Several studies have identified the enzyme type I dehydroquinase (DHQ1, 3-dehydroquinate dehydratase, EC 4.2.1.10) as a promising target for anti-virulence drug development. DHQ1 catalyzes the reversible dehydratation of 3-dehydroquinic acid (1) to 3-dehydroshikimic acid (2), which is the third step in the shikimic acid pathway. It follows a covalent catalysis mechanism with the formation of transient Schiff base species´ between the ketone moiety of the substrate and the ɛ-amino group of a catalytic lysine residue (K160/K170 in Sa-DHQ1 and St-DHQ1, respectively), which are finally hydrolyzed to regenerate the enzyme. An essential histidine residue (H133/H143 in Sa-DHQ1 and St-DHQ1, respectively), is also involved in the formation/hydrolysis of the Schiff base intermediates.

Herein we report the synthesis of compounds 6–7 in which enhancement of the electrophilicity of an endocyclic carbon atom in the ligand towards covalent modification is attempted by direct introduction of the amino functionality into the quinate scaffold. These compounds are substrate analogs in which the carbonyl group at C3 has been replaced by a hydroxyamino and an amino group with R configuration (compounds 6 and 7, respectively). Compound 6 was found to be a time-dependent irreversible inhibitor of the two enzymes with K I values of 90 ± 8 and 130 ± 12 µM and k inact values of 8 ± 1 and 13 ± 1 ms−1 against Sa-DHQ1 and St-DHQ1, respectively. The two adducts Sa-DHQ1/6 and St-DHQ1/6 crystallized as dimers with two molecules in the asymmetric unit (namely chains A and B) and were solved at a resolution of 1.65 and 1.90 Å, respectively. Unbiased, calculated electron-density maps showed clear electron density for the ligand covalently bonded to the catalytic lysine residue (K160/K170 in Sa-DHQ1 and St-DHQ1, respectively) via an amine, which is visible in the two chains. Remarkably, among all the lysine residues present in the two enzymes (13 for Sa-DHQ1 and 11 for St-DHQ1), only the catalytic lysine residue is modified by the ligand. Surprisingly, no electron density for the tertiary hydroxyl group in position C1 was identified in the two enzyme adducts. Dehydration involving the C1–C2 bond took place to give a shikimate-like core, perhaps after covalent linkage at the C3 position in 6 via a similar mechanism to that observed for the natural substrate. Importantly, no cleavage of the amine bond promoted by the ligand was observed. Thus, compound 6 provides non-labile enzyme adducts by avoiding the intrinsic Schiff base hydrolysis performed by the enzyme. Finally, the active site of both adducts is closed by the substrate-covering loop, thus protecting the catalytic pocket from the water environment.

>MTHVEVVATIAPQLYIEETLIQKINHRIDAIDVLELRIDQIENVTVNQVAEMITKLKVMQDSFKLLVTYRTKLQGGYGQFTNDLYLNLISDLANINGIDMIDIEWQADIDIEKHQRIITHLQQYNKEVVISHHNFESTPPLDELQFIFFKMQKFNPEYVKLAVMPHNKNDVLNLLQAMSTFSDTMDCKVVGISMSKLGLISRTAQGVFGGALTYGCIGEPQAPGQIDVTDLKAQVTLY[2x]>MISGLSHITLIVKDLNKTTAFLQNIFNAEEIYSSGDKTFSLSKEKFFLIAGLWICIMEGDSLQERTYNHIAFQIQSEEVDEYTERIKALGVEMKPERP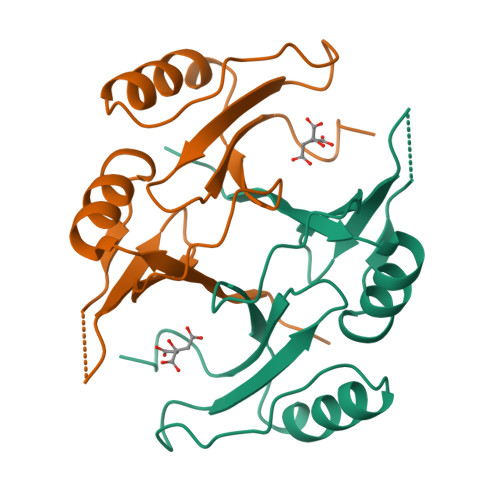RVQGEGRSIYFYDFDNHLFELHAGTLEERLKRYHE[2x]> GIDPFTKHGQKECDNALRQLETVRELLENPVQPINDMSYFGCLDSVMENSKVLGEAMTGISQNAKNGNLPEFGDAIATASKALCGFTEAAAQAAYLVGVSDPNSQAGQQGLVEPTQFARANQAIQMACQSLGEPGCTQAQVLSAATIVAKHTSALCNSCRLASARTANPTAKRQFVQSAKEVANSTANLVKTIKALDGDFTEENRAQCRAATAPLLEAVDNLSAFASNPEFSSVPAQISPEGRAAMEPIVISAKTMLESAGGLIQTARALAVNPRDPPRWSVLAGHSRTVSDSIKKLITSMRDKAPGQL;> PELDDILYHVKGMQRIVNQWSEK

Talin plays a key role in coupling integrin receptors to the actomyosin contractile machinery, while deleted in liver cancer 1 (DLC1) is a Rho GAP that binds talin and regulates Rho, and therefore actomyosin contractility. Talin comprises an N-terminal FERM domain (∼50 kDa) that binds to and activates integrins, connected to a large flexible rod (∼200 kDa) that interacts with multiple ligands, including vinculin and F-actin (Calderwood et al., 2013). The talin rod constitutes a force-sensing module that regulates the assembly and maturation of adhesion complexes, and is composed of 13 four- and five-helical bundles connected by short linkers, forming an extended flexible chain (Goult et al., 2013b). The DLC1 binding site in talin has been mapped by deletion analysis to the four-helix R8 domain (Li et al., 2011) that forms a unique protrusion in the C-terminal part of the rod that is otherwise composed of a linear chain of five-helix bundles (Gingras et al., 2010).

For these reasons, we used the longer DLC1 fragment for solution binding studies and the shorter fragment for crystallization experiments. We crystallized a complex of DLC1(467–489) with the talin R7R8 fragment, the structure of which we previously determined in the free form (Gingras et al., 2010), and solved the structure of the complex by molecular replacement (statistics in Table 1). As in the free form, the R7R8 talin rod fragment adopts a unique fold where the R8 four-helix bundle is inserted into the loop connecting helices α3 and α4 of the R7 five-helix bundle. Individually, the structures of R7 and R8 in the DLC1 complex are nearly identical to that of the free form (root-mean-square deviation [RMSD] 0.35 Å and 1.75 Å, respectively), the main difference being the relative orientation of the two domains. As expected from sequence analysis and NMR data, the DLC1 peptide forms an α helix that interacts only with the talin R8 domain. The DLC1 helix docks into the hydrophobic groove formed by helices α2 and α3 of talin R8, forming a canonical left-handed anti-parallel triple-helix coiled-coil arrangement. At the N-terminal end of the DLC1 helix, corresponding to the LD motif, residues L469, I472, L473, and V476 are embedded between the hydrophobic side chains of L1492 of the R8 α2 helix, and V1540, K1541, and I1543 of the α3 helix in a “knobs-into-holes” arrangement typical for the coiled-coil packing, creating a small hydrophobic core. The negatively charged DLC1 residue D470 that is conserved within LD motifs (the “D” residue) makes direct contact with the positively charged side chain of K1544 in R8. The polar side chains of Q480 and N484 in DLC1 (positions “e” and “b” of the heptad repeat) make contacts with the matching polar groups of N1534 and N1538 at the edge of the R8 α2-α3 hydrophobic patch, creating a polar ridge. This ridge is extended by charge contacts between E488 of DLC1, which is wedged between the positively charged groups R1523 and K1530 of R8.>MDAAIRGNDVIFVLKTIGVPSACRQNEDPRFVEAFKCDELERYIDNNPECTLFESLRDEEAYSIVRIFMDVDLDACLDEIDYLTAIQDFIIEVSNCVARFAFTECGAIHENVIKSMRSNFSLTKSTNRDKTSFHIIFLDTYTTMDTLIAMKRTLLELSRSSENPLTRSIDTAVYRRKTTLRVVGTRKNPNCDTIHVMQPPHDNIEDYLFTYVDMNNNSYYFSLQRRLEDLVPDKLWEPGFISFEDAIKRVSKIFINSIINFNDLDENNFTTVPLVIDYVTPCALCKKRSHKHPHQLSLENGAIRIYKTGNPHSCKVKIVPLDGNKLFNIAQRILDTNSVLLTERGDHIVWINNSWKFNSEEPLITKLILSIRHQLPKEYSSELLCPRKRKTVEANIRDMLVDSVETDTYPDKLPFKNGVLDLVDGMFYSGDDAKKYTCTVSTGFKFDDTKFVEDSPEMEELMNIINDIQPLTDENKKNRELYEKTLSSCLCGATKGCLTFFFGETATGKSTTKRLLKSAIGDLFVETGQTILTDVLDKGPNPFIANMHLKRSVFCSELPDFACSGSKKIRSDNIKKLTEPCVIGRPCFSNKINNRNHATIIIDTNYKPVFDRIDNALMRRIAVVRFRTHFSQPSGREAAENNDAYDKVKLLDEGLD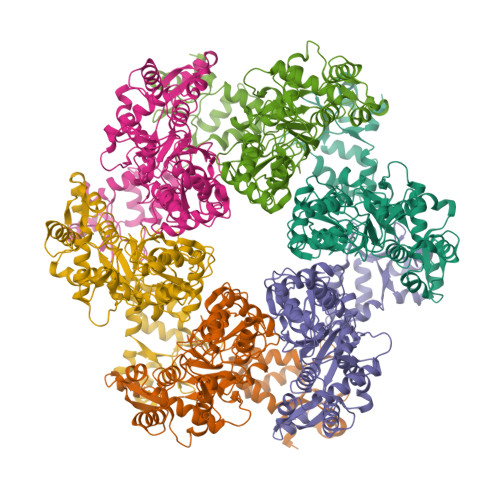GKIQNNRYRFAFLYLLVKWYKKYHIPIMKLYPTPEEIPDFAFYLKIGTLLVSSSVKHIPLMTDLSKKGYILYDNVVTLPLTTFQQKISKYFNSRLFGHDIESFINRHKKFANVSDEYLQYIFIEDISSP[6x]> ESDTGLWLHNKLGATDELWAPPSIASLLTAAVIDNIRLCFHGLSSAVKLKLLLGTLHLPRRTVDEMKGALMEIIQLASLDSDPWVLMVADILKSFPDTGSLNLELEEQNPNVQDILGELREKVGECEASAMLPLECQYLNKNALTTLAGPLTPPVKHFQLKRKPKSATLRAELLQKS;> GEITSVSTACQQLEVFSRVLRTSLATILDGGEENLEKNLPEFAKMVCHGEHTYLFAQAMMSVLAQEEQGGSAVRRIAQEVQRFAQEKGHDASQITLALGTAASYPRACQALGAMLSKGALNPADITVLFKMFTSMDPPPVELIRVPAFLDLFMQSLFKPGARINQDHKHKYIHILAYAASVVETWKKNKRVSINKDELKSTSKAVETVHNLCCNENKGASELVAELSTLYQCIRFPVVAMGVLKWVDWTVSEPRYFQLQTDHTPVHLALLDEISTCHQLLHPQVLQLLVKLFETEHSALDVMEQLELKKTLLDRMVHLLSRGYVLPVVSYIRKCLEKLDTDISLIRYFVTEVLDVIAPPYTSDFVQLFLPILENDSIAGTIKTEGEHDPVTEFIAHCKSNFIMVN

Promoter-proximal pausing also employs the negative elongation factor (NELF), which comprises the four subunits NELF-A, -B, -C (or its variant -D, which lacks nine N-terminal amino acid residues), and -E. NELF was identified as a complex that cooperates with DSIF to repress Pol II elongation. Here we show that regions of human NELF-A and NELF-C form a highly conserved core subcomplex with a novel fold. One side of this NELF-AC subcomplex exhibits a conserved binding face for single-stranded nucleic acids.

Bacterial co-expression of NELF subunit variants revealed that the N-terminal region of NELF-A could be co-purified with NELF-C. Limited proteolysis and co-expression analysis with truncated protein variants showed that the N-terminal residues 6–188 of human NELF-A and residues 183–590 of human NELF-C formed a stable subcomplex (‘NELF-AC’). The structure contained one NELF-AC heterodimer in the asymmetric unit and was refined to a free R-factor of 25.6% at 2.8Å resolution. The structure of human NELF-AC reveals a novel fold and an extended interface between the two NELF subunits. NELF-C consists of 22 α-helices (α1’-α22’) and a small two-stranded β-sheet (β1’-β2’, residues 367–379) that protrudes from the surface. The C-terminal half of NELF-C (helices α14’-α19’) forms three HEAT repeats (H1-H3). Subunit NELF-A forms a highly conserved helical ‘N-terminal domain’ (helices α1–α5, residues 6–110) that resembles the fold of the HIV integrase-binding domain present in human PC4 and SFRS1-interacting protein (PSIP1). Two invariant tryptophan side chains (W24 and W89) on the NELF-A N-terminal domain insert into largely conserved hydrophobic pockets of NELF-C. NELF-A helices α7 and α8 are buried in the NELF-C horseshoe. Overall, the heterodimer interface has a large surface area (3690 Å2), explaining the stability of the complex in 2 M sodium chloride (not shown). Analysis of the surface of the NELF-AC structure showed that the face opposite of where we detected NELF-BE crosslinks contains four positively charged patches (bottom view).> ATTLYLTRHGETKWNVERRMQGWQDSPLTEKGRQDAMRLGKRLEAVELAAIYTSTSGRALETAEIVRGGRLIPIYQDERLREIHLGDWEGKTH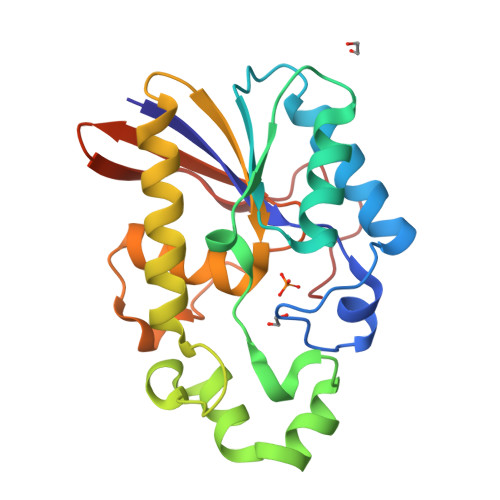DEIRQMDPIAFDHFWQAPHLYAPQRGERFCDVQQRALEAVQSIVDRHEGETVLIVTHGVVLKTLMAAFKDTPLDHLWSPPYMYGTSVTIIEVDGGTFHVAVEGDVSHIEEVKEV>[2x]MDNFFTEGTRVWLRENGQHFPSTVNSCAEGIVVFRTDYGQVFTYKQSTITHQKVTAMHPTNEEGVDDMASLTELHGGSIMYNLFQRYKRNQIYTYIGSILASVNPYQPIAGLYEPATMEQYSRRHLGELPPHIFAIANECYRCLWKRHDNQCILISGESGAGKTESTKLILKFLSVISQQSLELSLKEKTSCVERAILESSPIMEAFGNAKTVYNNNSSRFGKFVQLNICQKGNIQGGRIVDYLLEKNRVVRQNPGERNYHIFYALLAGLEHEEREEFYLSTPENYHYLNQSGCVEDKTISDQESFREVITAMDVMQFSKEEVREVSRLLAGILHLGNIEFITAGGAQVSFKTALGRSAELLGLDPTQLTDALTQRSMFLRGEEILTPLNVQQAVDSRDSLAMALYACCFEWVIKKINSRIKGNEDFKSIGILDIFGFENFEVNHFEQFNINYANEKLQEYFNKHIFSLEQLEYSREGLVWEDIDWIDNGECLDLIEKKLGLLALINEESHFPQATDSTLLEKLHSQHANNHFYVKPRVAVNNFGVKHYAGEVQYDVRGILEKNRDTFRDDLLNLLRESRFDFIYDLFEHVSSRNNQDTLKCGSKHRRPTVSSQFKDSLHSLMATLSSSNPFFVRCIKPNMQKMPDQFDQAVVLNQLRYSGMLETVRIRKAGYAVRRPFQDFYKRYKVLMRNLALPEDVRGKCTSLLQLYDASNSEWQLGKTKVFLRESLEQKLEKRREEE

Class X myosin has been found to be localized at the tips of filopodia, which are plasma membrane protrusions containing bundled actin that are necessary for cellular processes such as cell adhesion, migration, angiogenesis and the formation of cell–cell contacts. Myosin X is required for filopodia formation and extension. Myosin motors move along actin filaments via a series of conformational changes in the motor domain that are coupled with the sequential release of MgATP hydrolysis products, Pi and MgADP. These conformational changes in the motor domain are amplified by the myosin lever arm, which is comprized of the C-terminal subdomain of the motor domain (known as the converter) and an extended alpha helix length that varies with the myosin class12.

Given the surprising large step size that we measured for the myosin X dimers, we next evaluated whether the motor domain was capable of generating a larger angular swing than myosin V. We had previously shown that myosin VI has an unusual rearrangement of its converter domain in its pre-powerstoke state (PPS). This state in fact corresponds to the structure populated by myosin upon its re-attachment to the filament with a primed (pre-stroke) position for its lever arm. We thus crystallized the motor domain of myosin X in the pre-powerstroke state (with ADP vanadate bound) at 1.8 Å resolution, as well as that of the MD2IQ of myosin X at 3.1 Å resolution. The PPS structure differs in the orientation and position of the converter as compared with other plus-end myosins. Comparison of these PPS structures show that while the subdomains of the motor are totally conserved in position among the myosin PPS structures obtained to date, the myosin X converter is rotated compared with that of myosin Vc and other myosins. This is not due to a conformational change within the converter as found in myosin VI27. Instead, a sharper turn at the end of the SH1 helix, (at Gly672), allows formation of specific interactions between the converter and the Nter subdomain in particular with class-specific loops of this subdomain.> LELQEHCSLKPYNTFGIDVRARLLA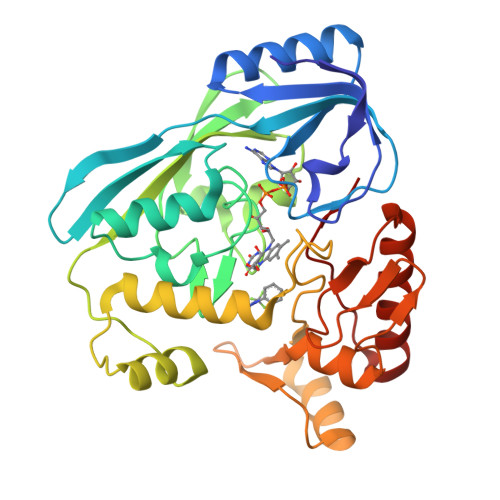HARDEADVREALALARERGLPLLVIGGGSNLLLTRDVEALVLRMASQGRRIVSDAADSVLVEAEAGEAWDPFVQWSLERGLAGLENLSLIPGTVGAAPMQNIGAYGVELKDVFDSLTALDRQDGTLREFDRQACRFGYRDSLFKQEPDRWLILRVRLRLTRRERLHLDYGPVRQRLEEEGIASPTARDVSRVICAIRREKLPDPAVLGNAGSFFKNPLVDATQAERLRQAFPDLVGYPQADGRLKLAAGWLIDKGGWKGFRDGPVGVHAQQALVLVNHGGATGAQVRALAERIQEDVRRRFGVELEPEPNLY>[2x]MGNKYRVRKNVLHLTDTEKRDFVRTVLILKEKGIYDRYIAWHGAAGKFHTPPGSDRNAAHMSSAFLPWHREYLLRFERDLQSINPEVTLPYWEWETDAQMQDPSQSQIWSADFMGGNGNPIKDFIVDTGPFAAGRWTTIDEQGNPSGGLKRNFGATKEAPTLPTRDDVLNALKITQYDTPP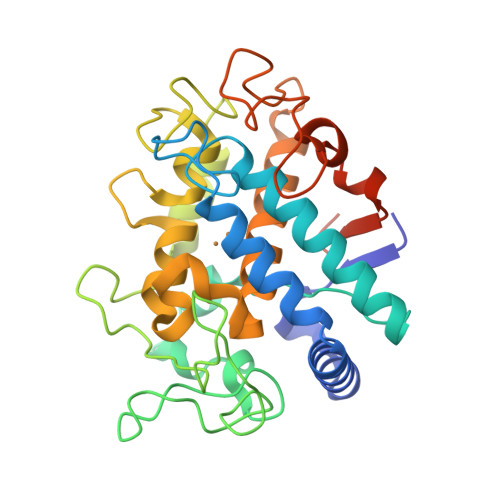WDMTSQNSFRNQLEGFINGPQLHNRVHRWVGGQMGVGPTAPNDPVFFLHHANVDRIWAVWQIIHRNQNYQPMKNGPFGQNFRDPMYPWNTTPEDVMNHRKLGYVYDIELRKSKRSSHHHHHH>MLGSGFKAERLRVNLRLVINRLKLLEKKKTELAQKARKEIADYLAAGKDERARIRVEHIIREDYLVEAMEILELYCDLLLARFGLIQSMKELDSGLAESVSTLIWAAPRLQSEVAELKIVAD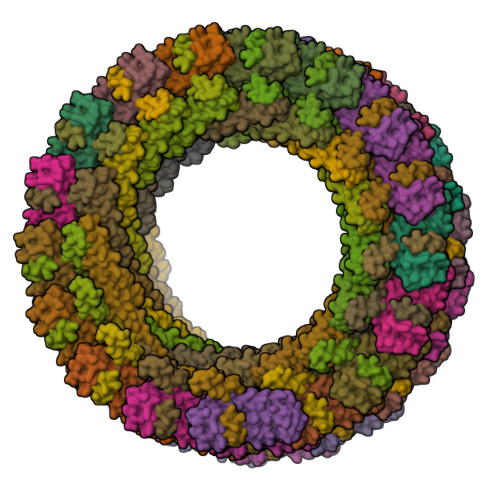QLCAKYSKEYGKLCRTNQIGTVNDRLMHKLSVEAPPKILVERYLIEIAKNYNVPYEPDSVVMAEAPPGVETDLIDVGFTDDVKKGGPGRGGSGGFTAPVGGPDGTVPMPMPMPMPMPSANTPFSYPLPKGPSDFNGLPMGTYQAFPNIHPPQIPATPPSYESVDDINADKNISSAQIVGPGPKPEASAKLPSRPADNYDNFVLPELPSVPDTLPTASAGASTSASEDIDFDDLSRRFEELKKKT[36x];>[36x]MSNMEKHLFNLKFAAKELSRSAKKCDKEEKAEKAKIEKAIQKGNMEVARIHAENAIRQKNQAVNFLRMSARVDAVAARVQTAVTMGKVTKSMAGVVKSMDATLKTMNLEKISALMDKFEHQFETLDVQTQQMEDTMSSTTTLTTPQNQVDMLLQEMADEAGLDLNMELPQGQTGSVGTSVASAEQDELSQRLARLRDQV>[2x]MGSSHHHHHHSSGENLYFQGHMLDWVDGRPAAELSVRDRGLAYGDGLFETLAVRAGTPRLLERHLARLEEGCRRLAIPLDTAAL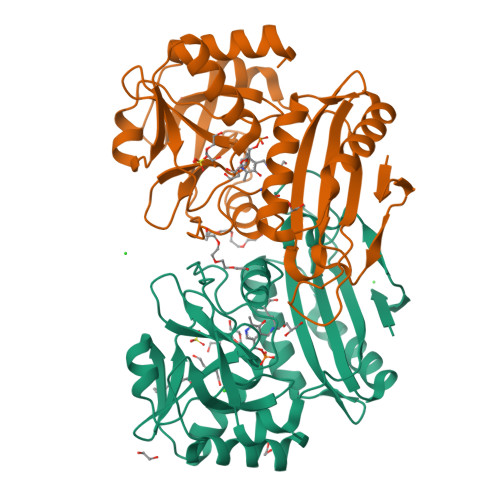RQELLAFCAALGDGVAKLIVTRGEGLRGYAPPAEASPRRILSGSPRPAYPERHWQQGVRLFACRTRLAEQPLLAGLKHLNRLEQVLARAEWSDAGHAEGLMLDVHERVVEGVFSNLLLVLDGTLVAPDLRRCGVAGVMRAELLERAEGIGVPLAIRDVSMAELATADEVFLCNSQFGIWPVRALDEHVWPVGELTRKLQDQLRDDLDF>[2x]MAHHHHHHSSGLEVLFQMDEFEEYRNPLTKRYASREMVCNFGEKRKVILWRQLWIWLAETQKEL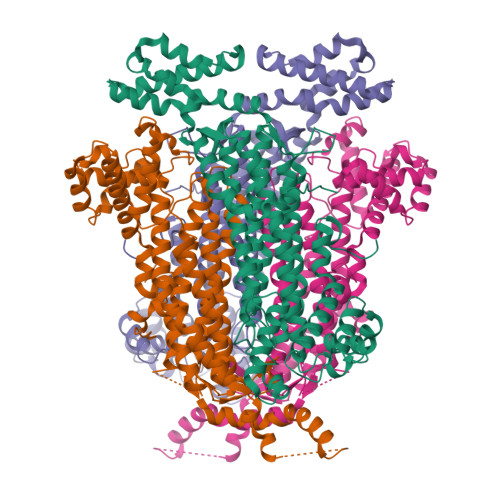GFDITDEQINEMKSQRDSVDFGTAAAEEKARRHDVMAHVYTFALACPKAAPIIHLGATSCFVGDNADLIMLKDGLNILLPKVARCIDRLAKKAMLHKSLICLARTHLQPAQPTTMGRRICMWIQDLLLDLENLERLKNHTIRFRGAKGAVGTQASFMDLFQGDHQKVIKLDEILTKKSGFQRSWCVTGQTYPRKVDIEITNALSNIGATVHKICTDIRLLSSFHEVEEPFETKQIGSSAMPYKRNPIRSERACSLARYLMHISTSMVSTVSVQWLERSLDDSAIRRIVLPEAFLAADACLTLLQNIAEGLIVYPMVMEANLNSELPFLVVERILVKMVSEGAANRQECHERLRKHSHEAAAEIKLKGLKNSLMDKLLNDYYFAPIHSLLPTVLDPSYMIGRAVEQVEVFLNTEVDPAIHSYKDCLALNSNITI>[2x]GAMDPASLEEMLTQAVQEADIEQVRQLLERGADANFQEEEWGWSPLHSAVQMDSEDLVALLLKHGADPCLRKRNGATPFIIAGITGNVRLLQLLLPNV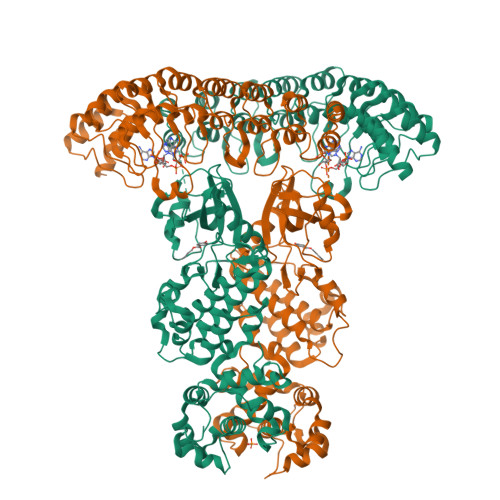EDVNECDVNGFTAFMEAAVYGRVEALRFLYENGADVNMHRKTKQDQERIRKGGATALMDAAEKGHVGVVTILLHAMKAEVDARDNMGRNALVYALLNPDDGKAKAITRLLLDHGADVNVRGEGSKTPLILAVERKNLDLVQMLLEQEQIEVNDTDREGKTALLLAVELRLEEIAKLLCHRGASTNCGDLVAIARRNYDSDLVKFLRLHKAGEDFRPPAENWKPQSSRWGEALKHLHRIWRPMIGKLKIFIDEEYKIADTAEGGIYLGLYEDQEVAVKRFSEGSTRGQQEVSCLQSSRANDNVVTFYGSESDGSCLHVCLALCEYTLQEHLANHRGDAVPNEEDESARNILSSLFKAIGELHRSGYSHQDLQPQNILIDSKNGTFLADFDKSIKWAEDPQKIKRDLEALGLLVLYVVKKGDISFETLKNQSFEEVIQGSPDEETRDLIHHLFHPGDNVEDRLSSLLAHPFFWSWESRYRTLRDVGNESDIKTRNQNSRILQLLQPGTSELSTSFAQWTTKIDSFVMEEMNAYYKKISKKKKAKHTNEGNLYQDTLGDLLKFIRNLGEHINEQKNKKMKSIIGEPSQYFQEKFPDLVMYVYTKLQNTEYMKHFPKTHNPNK>[2x]MSFETSEGMSRPGDNPNKLNAKPRQSARPKTRNSTAQSNQTMR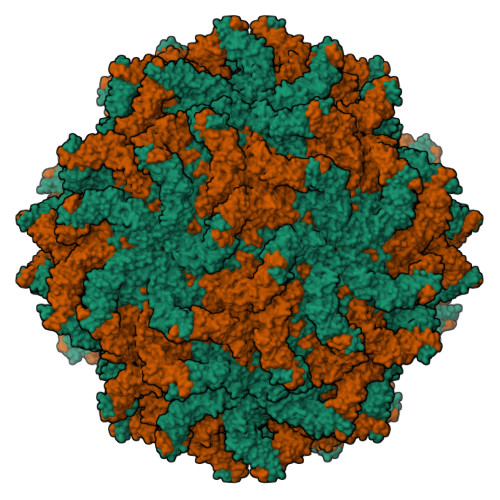LGWIDPLPQVDTIFPLGLEPNVESIPAGEVELDFNLPETIAKPFADTVTSVGDRIQLVDDDKENIATSIYGLSFFKAARQLYSTMLDHEKAVNQPLKAVYYDETPIPAHMSGALGIIGHMKTKVGDVLVKDAGVLFKRGTAAGVTKFSEIDNDKTWNLDCSKLVWADHSSLSMIKRLASEKISQLVKQRYRVTDAQGHVYSVSMPQLTDQALPDYYDSIPDVAPNSDQLRVLTAALQMSLAQFRNDELPHDEDRSDLLTTLDLLYADGAYEISALRDQFELLMARYTTDFKWRVESIFKVGPPPAGTTGYGAQTVSSTGNTARWQFPLSDADINIGYLFSPSKSFSLFPKMVGYSKRAREDASASFANSDAKKFYAD>[2x]GPGSMALTAEEETIVKTVHDFVEKQVKPVVRELEHANTYPEELIETMKEIGIFGLAIPEPYGFGAVSMPCYVQVAEELARGWMSLAGAMGGHTVVSKLLLLFGTEEQKQKYLPRMATGELRATMALTEPGGGSDLQAMRTVARRDGDDYVINGSKTWISNA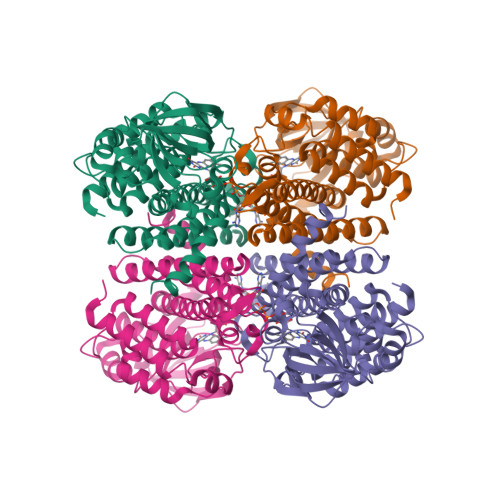RRSDLVALMCKTDPDAQPAHKGVSILLVEKVPGFDVSRDLPKLGYKGVESCELNFTDARVPVSSLLGDDEGRGFAQMMKGLEVGRLQVAARATGVARAAFEDALRYSQERESFGKPIWQHQSVGNMLADMGTKLYAARSLLLSAAEKFDAGQRCDMEAGMAKLFASETAMQIALDAVRVHGGYGYSTEYDVERYFRDAPLMIVGEGTNEIQRNVIAKQLVARGGLDI>MIDMYLYDDNEESQVQFVGFVGEHSRYDLMLVHTNRHYGKTLVLNMQTNKFGIIGTDDLKEEGYIAHILGVNAEEGDEI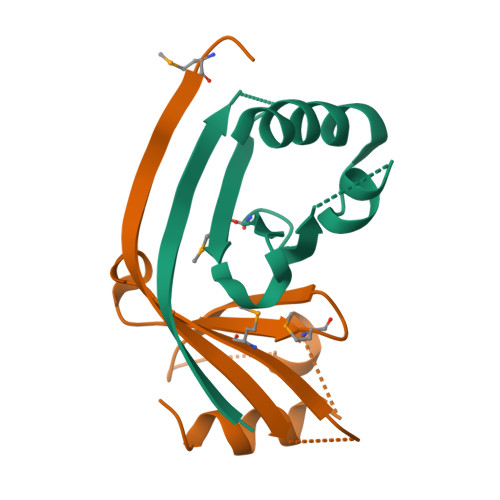TEYLNEVIHLEHHHHHH[10x]> MLSVLRPFPSPLLSRHGIDLDFPLLAGCLALLGLGLVMVTSASSEVAAAQSGNPLYFSVRHLIYLVIGLISCGLTMMVPMATWQRWGWKLLLVAFGLLVLVITPGIGREVNGSMRWIGFGLFNIQPSEIAKVCVVIFMAGYLIRRQQEVRESWMGFFKPFVVLLPMAGLLLREPDFGATVVMMGAAAAMLFLGGVGLFRFGLMVLLAVGAVVLLIQTQPYRMARLTNFTDPWADQFGAGYQLSQALIAFGRGGWLGMGLGNSIQKQFYLPEAHTDFVFAVLAEELGIVGALATVALFVFVSLRALYIGIWAEQAKQFFSAYVAYGLAFLWIGQFLINIGVNVGLLPTKGLTLPFLSYGGSSLVICCACLGMLLR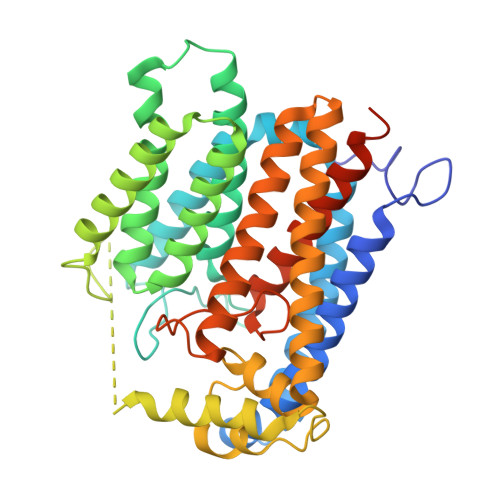IEWERRTHLGSEEYEFNEEDFADER>[8x]GHAGTTYIFSKGGGQITYKWPPNDRPSTRADRLAIGFSTVQKEAVLVRVDSSSGLGDYLELHIHQGKIGVKFNVGTDDIAIEES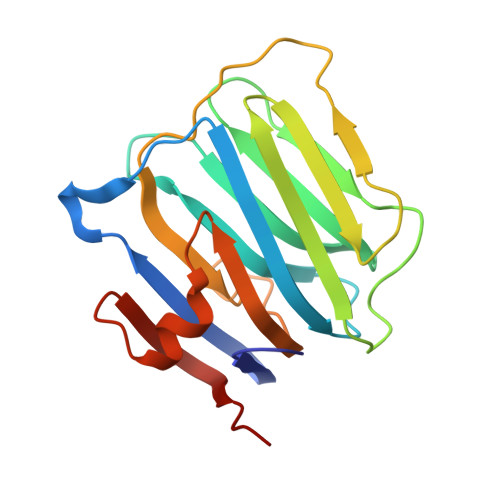NAIINDGKYHVVRFTRSGGNATLQVDSWPVIERYPAGRQLTIFNSQATIIIGGKEQGQPFQGQLSGLYYNGLKVLNMAAENDANIAIVGNVRLVGEVP> GASPSAQELKEQGNRLFVGRKYPEAAACYGRAITRNPLVAVYYTNRALCYLKMQQHEQALADCRRALELDGQSVKAHFFLGQCQLEMESYDEAIANLQRAYSLAKEQRLNFGDDIPSALRIAKKKRWNSIEERR;> XPCYEAWVLCEYX

Here, we report a general and rapid method for discovering α-helically constrained (Helicon) polypeptides that cooperatively induce the interaction between two target proteins without relying on previously known binders or an intrinsic affinity between the proteins. We show that Helicons are capable of binding every major class of E3 ubiquitin ligases, which are of great biological and therapeutic interest but remain largely intractable to targeting by small molecules. In addition to possessing increased stability and membrane permeability, Helicons are capable of binding large, flat protein surfaces that are inaccessible to targeting by small molecules, and Helicons have been developed to target a range of PPI targets in cells and in vivo. Characterizing Helicon-E3 co-structures and mechanisms of action, we identified new binding sites for α-helices on the E3 surfaces, as well as potential probes of the disease-linked E3, WWP123,24, highlighting the generality of our approach against this therapeutically important target class.

We performed screens of the naive phage library to identify Helicons that bind MDM2 and CHIP. Among the resulting hits, we validated CHIP-binding Helicons H317 and H318 from C80, including by x-ray crystallography to examine binding to their E3 presenters. Surprisingly, while Helicons H317 and H318 belong to the same cluster, we noted several differences in the co-structures with CHIP, reflecting unique conformational changes and binding surfaces revealed by the Helicons. For instance, the side chain of Glu9 in H317 directly interacts with Lys30 of CHIPTPR while Glu10 from H318 does not. As a proof of concept, we selected hit clusters for the RING/U-Box family E3s CHIP and MDM2, including those exemplified by H319 for MDM2 and H317 and H318 for CHIP, and designed focused libraries by fixing the conserved binding residues and diversifying the surface-exposed Helicon residues. Screens with the CHIP-based trimerizer library identified several CHIP-dependent PPIA clusters, including C86, C88, C89, and C94. Helicon H326 from C88 could promote ternary complex formation between CHIP and PPIA as shown by TR-FRET, and this was abolished by unlabeled CsA and diminished by the CHIP-binder H318 described in Fig. 3c, suggesting that the complex forms via the CsA-binding site of PPIA and the H318-binding site of CHIP. As expected, an unlabeled YAP1 fragment could also disrupt the interaction. Finally, we confirmed that while H321 and H322 do not interact with TEAD4 alone, they did show weak binding affinity to CHIP, at a higher EC50 than the CHIP-binder H318 characterized in Fig. 3c.>MSLKITEVKAHALSTPIPERMRVESGAGLKLNRQMILVEVRTDEGVTGVGSPSGPYDLAVLKRAIEDVIGPQLIGEDPANINYLWHKVFHGEVSRNLGHRSVGIAAMSGVDIALWDLKGRAMNQPIYQLLGGKFHTRGVRAYASSIYWDLTPDQAADELAGWVEQGFTAAKLKVGRAPRKDAANLRAMRQRVGADVEILVDANQSLGRHDALAMLRILDEAGCYWFEEPLSIDDIEGHRILRAQGTPVRIATGENLYTRNAFNDYIRNDAIDVLQADASRAGGITEALAISASAASAHLAWNPHTFNDIITVAANLHLVAASPHPAMFEWDITHNDLM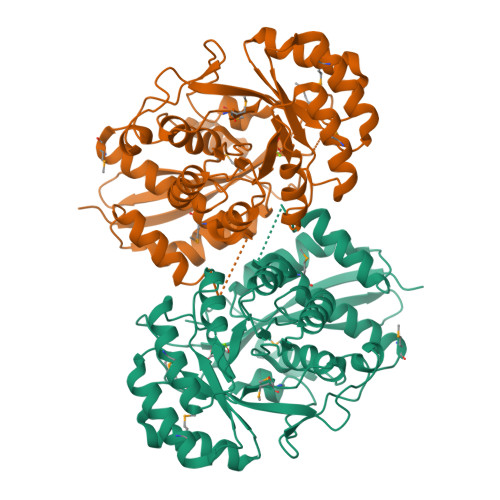TRLASYDLKLENGLVQPPQGPGLGFEIDWDFVAAHAWKGEPAIGAGHGMKKEGHHHHHH[2x]5-HYDROXYPENTANAL | C5 H10 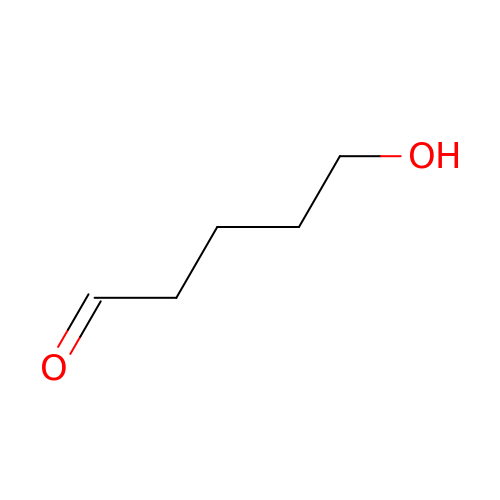O2 | CNRGMQRNYAIBTN-UHFFFAOYSA-N> PISPIETVPVKLKPGMDGPKVKQWPLTEEKIKALVEICTEMEKEGKISKIGPENPYNTPVFAIKKKDSTKWRKLVDFRELNKRT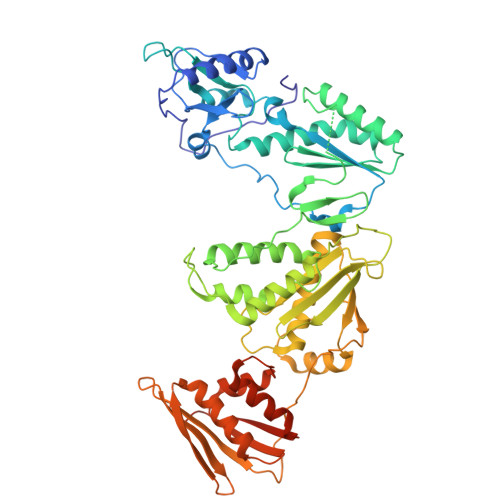QDFWEVQLGIPHPAGLKKKKSVTVLDVGDAYFSVPLDEDFRKYTAFTIPSINNETPGIRYQYNVLPQGWKGSPAIFQSSMTKILEPFKKQNPDIVIYQYMDDLYVGSDLEIGQHRTKIEELRQHLLRWGLTTPDKKHQKEPPFLWMGYELHPDKWTVQPIVLPEKDSWTVNDIQKLVGKLNWASQIYPGIKVRQLCKLLRGTKALTEVIPLTEEAELELAENREILKEPVHGVYYDPSKDLIAEIQKQGQGQWTYQIYQEPFKNLKTGKYARMRGAHTNDVKQLTEAVQKITTESIVIWGKTPKFKLPIQKETWETWWTEYWQATWIPEWEFVNTPPLVKLWYQLEKEPIVGAETFYVDGAANRETKLGKAGYVTNKGRQKVVPLTNTTNQKTELQAIYLALQDSGLEVNIVTDSQYALGIIQAQPDKSESELVNQIIEQLIKKEKVYLAWVPAHKGIGGNEQVDKLVSAGIRKIL>MFEGSITALVTPFADDRIDEVALHDLVEWQIEEGSFGLVPCGTTGESPTLSKSEHEQVVEITIKTANGRVPVIAGAGSNSTAEAIAFVRHAQNAGADGVLIVSPYYNKPTQEGIYQHFKAIDAASTIPIIVYNIPGRSAIEIHVETLARIFEDCPNVKGVKDATGNLLRPSLERMACGEDFNLLTGEDGTALGYMAHGGHGCISVTANVAPALCADFQQACLNGDFAAALKLQDRLMPLHRALFLETNPAGAKYA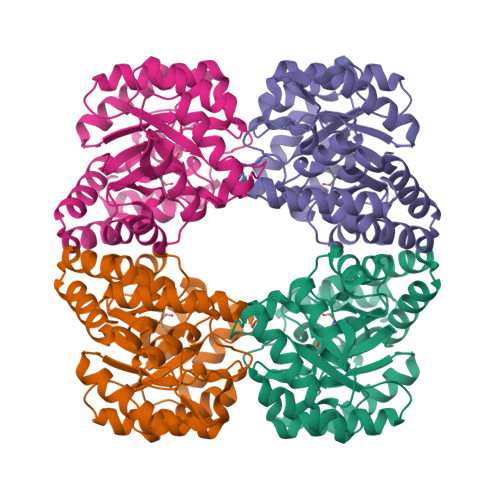LQRLGRMRGDLRLPLVTISPSFQEEIDDAMRHAGILL[2x]> FACKTANGTAIPIGGGSANVYVNLAPVVNVGQNLVVDLSTQIFCHNDYPETITDYVTLQRGSAYGGVLSNFSGTVKYSGSSYPFPTTSETPRVVYNSRTDKPWPVALYLTPVSSAGGVAIKAGSLI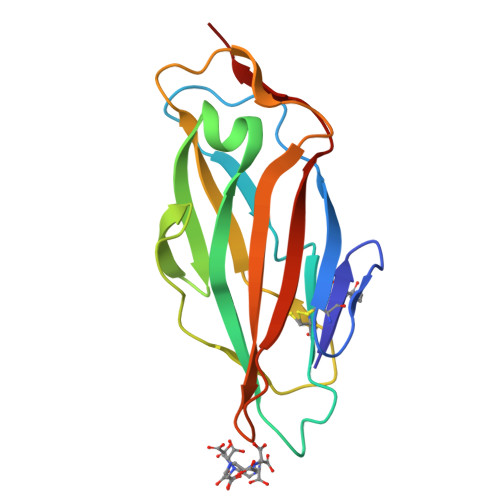AVLILRQTNNANSDDFQFVWNIYANNDVVVPT> MVSASQRTTSTATGDEWWAKCKQVDVLDSEMSYYDSDPGKHKNTVIFLHGNPTSSYLWRNVIPHVEPLARCLAPDLIGMGKSGKLPNHSYRFVDHYRYLSAWFDSVNLPEKVTIVCHDWGSGLGFHWCNEHRDRVKGIVHMESVVDVIESWDEWPDIEEDIALIKSEAGEEMVLKKNFFIERLLPSS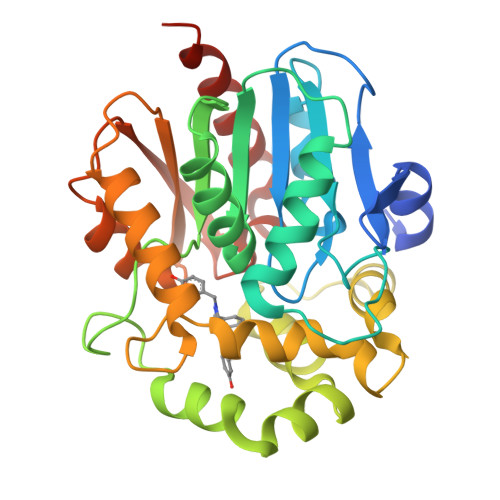IMRKLSEEEMDAYREPFVEPGESRRPTLTWPREIPLVKGGKPDVIEIVKSYNKWLSTSKDIPKLFINADPGFFSNAIKKVTKNWPNQKTVTVKGLHFLQEDSPEEIGEAIADFLNELTKHHHHHH>MDKLAVLYAEHIATLQQRTRTITEREGLEGLVIHSGQAKRQFLDWMYYPFKVNPQFKAWLPVIDNPHCWIVVDGASKPKLIFYRPVDFWHKVPDEPRDFWAEYFDIELLVQPDQVEKLLPYDKANYAYIGEYLEVAQALGFSIMNPEPV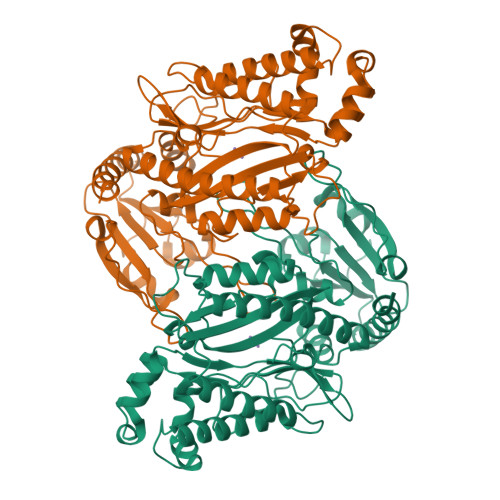MNYLHFHRAYKTQYELECLRQANRIAVEGHKAARDTFFNGGSEFDIQHAYLMATRQSENEMPYGNIVALNENCAIYLYTHFEPTAPHTHHSFLIDAGANFNGYAADITRTYDFKKSGEFSDLIQVMTEHQIALGKALKPGLLYGELHLECHQRVAQVLSDFNIVKLPAADIVERGITSTFFPHGLGHHLGLQVIDMGGFMADESGTHQAPPEGHPFLRCTRLIEKNQVFTIEPGLYFIDSLLGDLAQTDNKQFINWEKVEEFKPFGGIRIEDNIIVHEDSLENMTRDLHLDLEHHHHHH[4x]>SMSARKRIVVGVAGGIAAYKACTVVRQLTEAGHSVRVVPTESALRFVGAATFEALSGNPVHTGVFTDVHEVQHVRIGQQADLVVIAPATADLLARAVAGRADDLLTATLLTARCPVLFAPAMHTEMWLHPATVDNVATLRRRGAVVLEPASGRLTGADSGPGRLPEAEEITTLAQLLLERADALPYDMAGVKALVTAGGTREPLDPVRFIGNRSSGKQGYAVARVLAQRGADVTLIAGNTAGLIDPAGVEMVHIGSATQLRDAVSKHAPDANVLVMAAAVADFRPAHVAAAKIKKGASEPSSIDLVRNDDVLAGAVRARADGQLPNMRAIVGFAAETGDANGDVLFHARAKLERKGCDLLVVNAVGENRAFEVDHNDGWLLSADGTESALEHGSKTLMATRIVDSIAAFLKSQDG[4x]

However, in the vast majority of prokaryotes, including M. tuberculosis, CoaB and CoaC are encoded by a single gene to produce a fused bifunctional enzyme (CoaBC). CoaBC converts 4′-phosphopantothenate to 4′-phosphopantetheine in three steps. The product of CoaB is then decarboxylated by CoaC, an enzyme of the homo-oligomeric flavin-containing decarboxylase (HFCD) protein family, to 4′-phosphopantetheine. Transcriptional silencing of individual genes of the CoA biosynthetic pathway of this pathogen identified CoaBC as uniquely bactericidal within the CoA pathway, highlighting it as a good candidate for drug discovery.

We therefore set out to obtain a full-length structure of a mycobacterial CoaBC and we successfully solved the MsmCoaBC structure, which shares very high sequence identity with the M. tuberculosis orthologue (86% full-length, 84% CoaB enzyme) and hence is a valuable tool for studying M. tuberculosis CoaBC. Here we report the structure of the bifunctional CoaBC of M. smegmatis at 2.5 Å. The final model (residues 2–412) covers both CoaC and CoaB, but densities for several residues in three loop regions in CoaB are not observed (residues 290–298, 336–342, 363–376). The N-terminal CoaC of MsmCoaBC (residues 1–179) forms the same type of dodecameric arrangement seen in other HFCD family proteins, such as the peptidyl-cysteine decarboxylase EpiD18, and it sits at the core of the dodecamer with the two domains connected through a small loop region (residues 180–189) that tightly interacts with both. The active site of CoaC sits at the interface between two protomers of one CoaC trimer and a protomer of an adjacent CoaC trimer with the FMN site facing inwards towards the hollow centre of the dodecamer. Each CoaB of MsmCoaBC (residues 190–414) dimerises with a CoaB belonging to an adjacent trimer. The full protein resembles a tetrahedron with CoaB dimers positioned at the six edges and CoaC trimers at the four vertices. The shortest distance between a pair of CoaB and CoaC active sites is ~30 Å. The absence of dimerisation for the MsmCoaB when expressed alone suggests that the interactions between CoaC and CoaB in M. smegmatis, and likely all other Mycobacteriaceae, are fundamental for CoaB dimerisation and activity. The organisation of CoaBC is similar to other HFCD family proteins but unique in the sense that it contains more than one domain and highlights how the arrangement of the fused enzymes is essential for mycobacterial CoaB dimerisation and function.>QEQVAPPKDPAAALEDHKTRTDNRYEPSLDNLAQQDVAAPGAPEGVSALSDAQYNEANKIYFERCAGCHGVLRKGATGKALTPDLTRDLGFDYLQSFITYGSPAGMPNWGTSGELSAEQVDLMANYLLLDPAAPPEFGMKEMRESWKVHVAPEDRPTQQENDWDLENLFSVTLRDAGQIALIDGATYEIKSVLDTGYAVHISRLSASGRYLFVIGRDGKVNMIDLWMKEPTTVAEIKIGSEARSIETSKMEGWEDKYAIAGAYWPPQYVIMDGETLEPKKIQSTRGMTYDEQEYHPEPRVAAILASHYRPEFIVNVKETGKILLVDYTDLDNLKTTEISAERFLHDGGLDGSHRYFITAANARNKLVVIDTKEGKLVAIEDTGGQTPHPGRGANFVHPTFGPVWATSHMGDDSVALIGTDPEGHPDNAWKILDSFPALGGGSLFIKTHPNSQYLYVDATLNPEAEISGSVAVFDIKAMTGDGSDPEFKTLPIAEWAGITEGQPRVVQGEFNKDGTEVW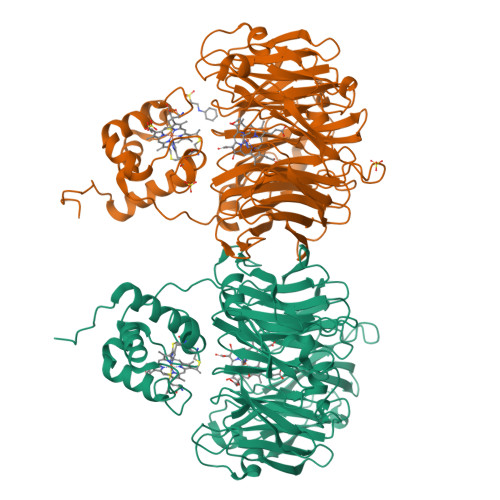FSVWNGKDQESALVVVDDKTLELKHVIKDERLVTPTGKFNVYNTMTDTY[2x]>MEPAMEPETLEARINRATNPL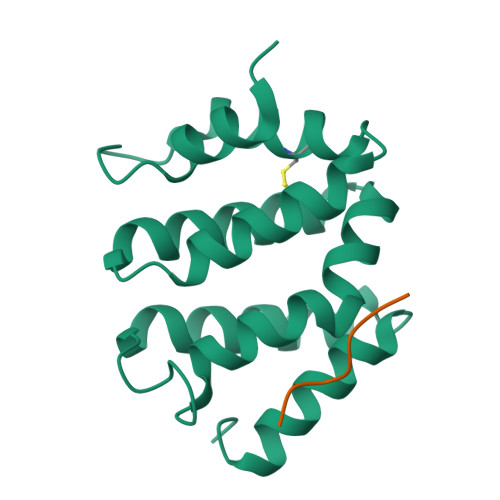NKELDWASINGFCEQLNEDFEGPPLATRLLAHKIQSPQEWEAIQALTVLETCMKSCGKRFHDEVGKFRFLNELIKVVSPKYLGSRTSEKVKNKILELLYSWTVGLPEEVKIAEAYQMLKKQGIVKS[2x];> HDDFADDISLLK[[O-PHOSPHONO-N-ACETYL-TYROSINYL]-GLUTAMYL-3[CYCLOHEXYLMETHYL]ALANINYL]-AMINE 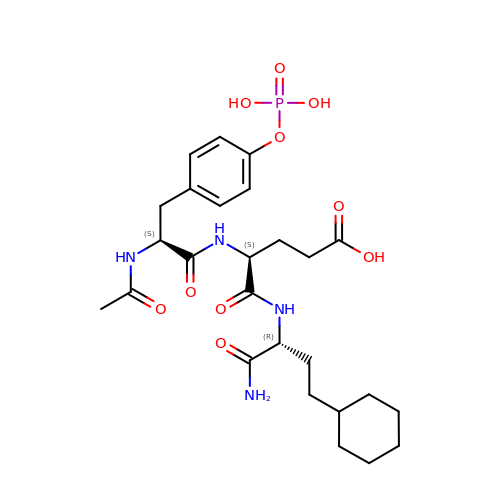| C26 H39 N4 O10 P | MYZLOAXXVDGNMQ-FSSWDIPSSA-N3-{[(4S)-2-amino-4-methyl-6-oxo-4-(propan-2-yl)-5,6-dihydropyrimidin-1(4H)-yl]methyl}-5-fluoro-N-[(1S)-1-phenylethyl]benzamide | C24 H29 F N4 O2 | 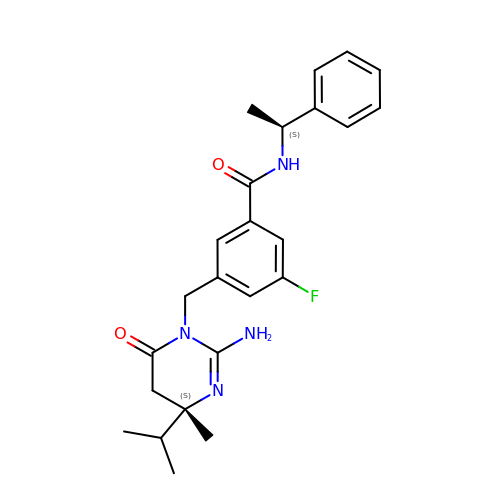PGSGWIDQXZCHJL-FYSMJZIKSA-N> GSHMASMTGGQQMGRGSMSLTEEKPIRPIANFSPSIWGDQFLIVDNQVEQGVEQIVKDLKKEVRQLLKEALDIPMKHANLLKLVDEIQRLGISYLFEQEIDHALQHIYETY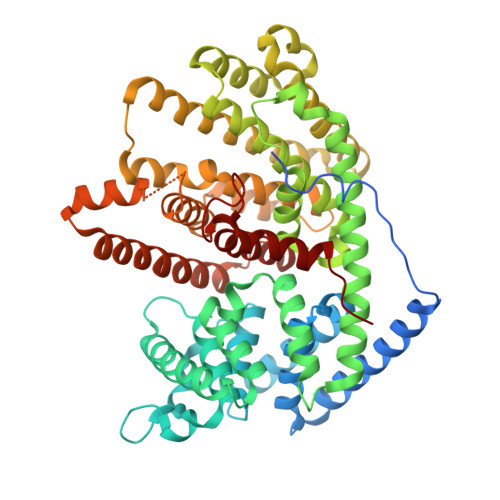GDNWSGDRSSLWFRLMRKQGYFVTCDVFNNHKDESGVFKQSLKNHVEGLLELYEATSMRVPGEIILEDALVFTQSHLSIIAKDTLSINPALSTEIQRALKKPLWKRLPRIEAVQYIPFYEQQDSHNKTLIKLAKLEFNLLQSLHREELSQLSKWWKAFDVKNNAPYSRDRIVECYFWALASRFEPQYSRARIFLAKVIALVTLIDDIYDAYGTYEELKIFTEAIERWSITCLDMIPEYMKPIYKLFMDTYTEMEEILAKEGKTNIFNCGKEFVKDFVRVLMVEAQWLNEGHIPTTEELDSIAVNLGGANLLTTTCYLGMSDIVTKEAFEWAVSEPPLLRYKGILGRRLNDLAGHKEEQERKHVSSSVESYMKEYNVSEEYAKNLLYKQVEDLWKDINREYLITKTIPRPLLVAVINLVHFLDVLYAEKDNFTRMGEEYKNLVKSLLVYPMSI>TELTKCKVSHAIKDIDGYQGISLLEWACVLFHTSGYDTQAVVNDNGSTEYGLFQISDRFWCKSSEFPESENICGISCDKLLDDELDDDIACAKKILAIKGIDYWKAYKPMCSEKLEQWRCEKP[2x];>ASMTGGQQMGRGSSLTACPEESPLLVGPMLIEFNIPVDLKLVEQQNPKVKLGGRYTPMDCISPHKVAIIIPFRNRQEHLKYWLYYLHPILQRQQLDYGIYVINQAGESMFNRAKLLNVGFKEALKDYDYNCFVFSDVDLIPMNDHNTYRCFSQPRHISVAMDKFGFSLPYVQYFGGVSALSK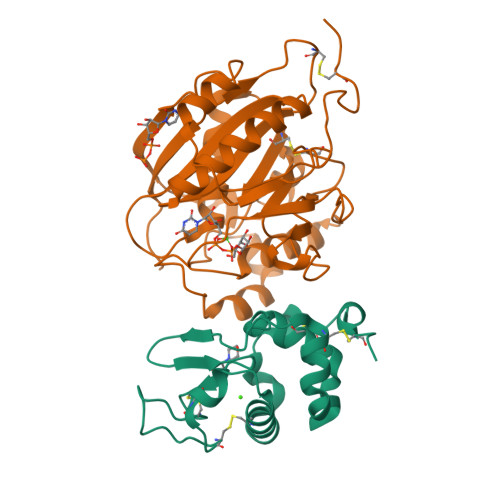QQFLSINGFPNNYWGWGGEDDDIYNRLAFRGMSVSRPNAVIGKTRHIRHSRDKKNEPNPQRFDRIAHTKETMLSDGLNSLTYMVLEVQRYPLYTKITVDIGTPS[2x]>MSHPDLNKLLELWPHIQEYQDLALKHGINDIFQDNGGKLLQVLLITGLTVLPGRAGNDAVDNAGQEYELKSINIDLTKGFSTHHHMNPVIIAKARQVPWIFAIYRGIAIEAIYRLEPKDLEFYYDKWERKWYSDGHKDINNPKIPVKYVME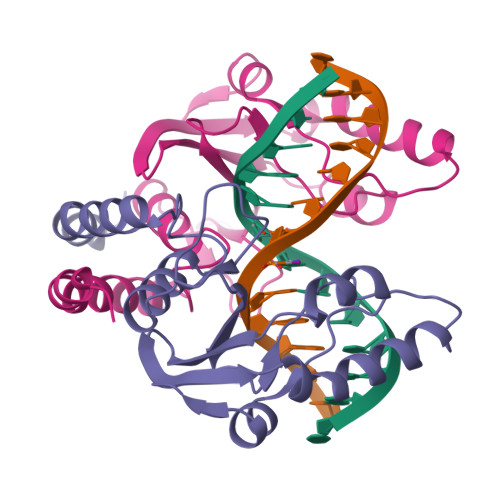HGTKIY[2x]> SMAAAEGPVGDGELWQTWLPNHVVFLRLREGLKNQSPTEAEKPASSSLPSSPPPQLLTRNVVFGLGGELFLWDGEDSSFLVVRLRGPSGGGEEPALSQYQRLLCINPPLFEIYQVLLSPTQHHVALIGIKGLMVLELPKRWGKNSEFEGGKSTVNCSTTPVAERFFTSSTSLTLKHAAWYPSEILDPHVVLLTSDNVIRIYSLREPQTPTNVIILSEAEEESLVLNKGRAYTASLGETAVAFDFGPLAAVPKTLFGQNGKDEVVAYPLYILYENGETFLTYISLLHSPGNIGKLLGPLPMHPAAEDNYGYDACAVLCLPC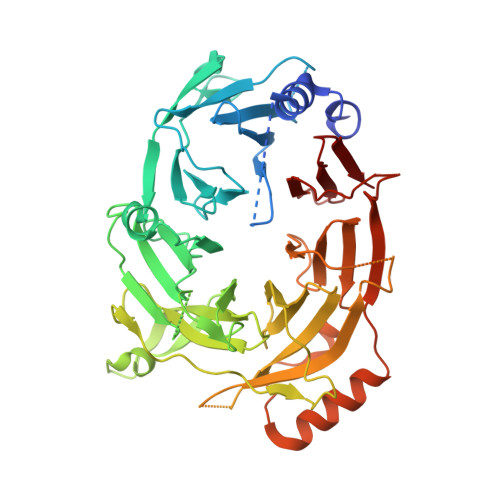VPNILVIATESGMLYHCVVLEGEEEDDHTSEKSWDSRIDLIPSLYVFECVELELALKLASGEDDPFDSDFSCPVKLHRDPKCPSRYHCTHEAGVHSVGLTWIHKLHKFLGSDEEDKDSLQELSTEQKCFVEHILCTKPLPCRQPAPIRGFWIVPDILGPTMICITSTYECLIWP>PPAVPQTFQVAHLHAPTGSGKSTKVPAAYAAQGYKVLVLNPSVAATLGFGAYMSKAHGIDPNIRTGVRTITTGGSITYSTYGKFLADGGCSGGAYDIIICDECHSTDSTTILGIGTVLDQAETAGARLVVLATATPPGSVTVPHPNIEEIGLSNNGEIPFYGKAIPIEAIKGGRHLIFCHSKKKCDELAAKLTGLGLNAVAYYRGLDVSVIPPIGDVVVVATDALMTGFTGDFDSVIDCNTCVTQTVDFSLDPTFTIETTTVPQDAVSRSQRRGRTGRGRSGIYRFVTPGERPSGMFDSSVLCECYDAGCAWYELTPAETSVRLRAYLNTPGLPVCQDHLEFWESVFTGLTHIDAHFLSQTKQAGDNFPYLVAYQATVCARA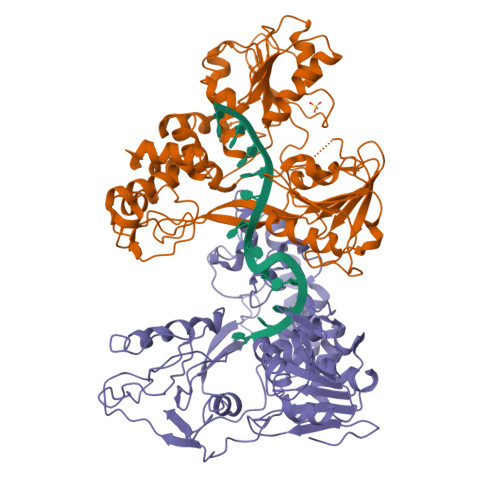QAPPPSWDQMWKCLIRLKPTLHGPTPLLYRLGAVQNEVILTHPITKYIMACMS[3x]>[3x]GRREQTHRAVFRFIPRHPDELELDVDDPVLVEAEEDDFWFRGFNMRTGERGVFPAFYAHAVPG;>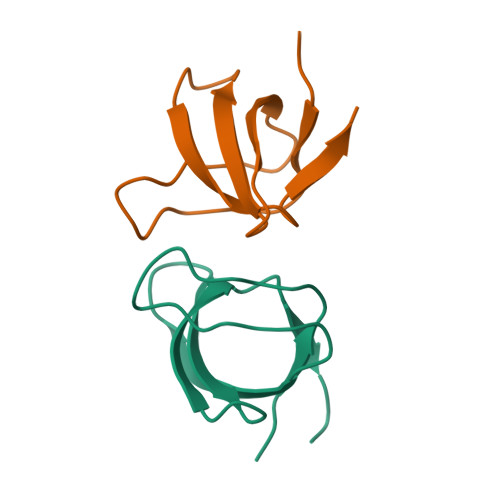 GHMEQTHRAIFRFVPRHEDELELEVDDPLLVELQAEDYWYEAYNMRTGARGVFPAYYAIEV> GMSFIEKMIGSLNDKREWKAMEARAKALPKEYHHAYKAIQKYMWTSGGPTDWQDTKRIFGGILDLFEEGAAEGKKVTDLTGEDVA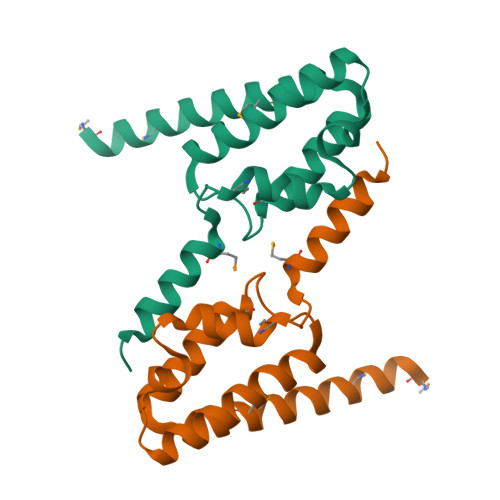AFCDELMKDTKTWMDKYRTKLNDSIGRD3,3',3''-[nitrilotris(methanediyl-1H-1,2,3-triazole-4,1-diyl)]tripropan-1-ol 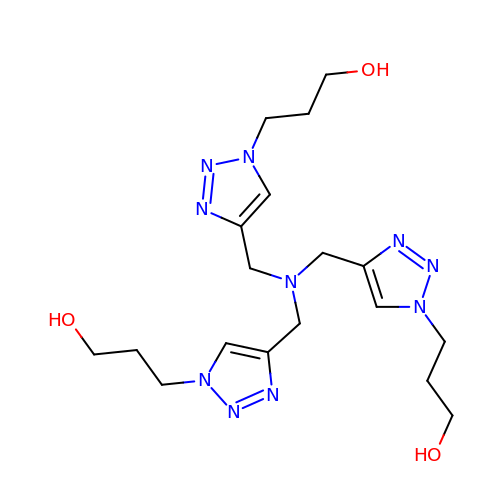| C18 H30 N10 O3 | VAKXPQHQQNOUEZ-UHFFFAOYSA-N>AEEWYFGKITRRESERLLLNPENPRGTFLVRESETTKGAYCLSVSDFDNAKGLNVKHYKIRKLDSGGFYITSRTQFSSLQQLVAYYSKHA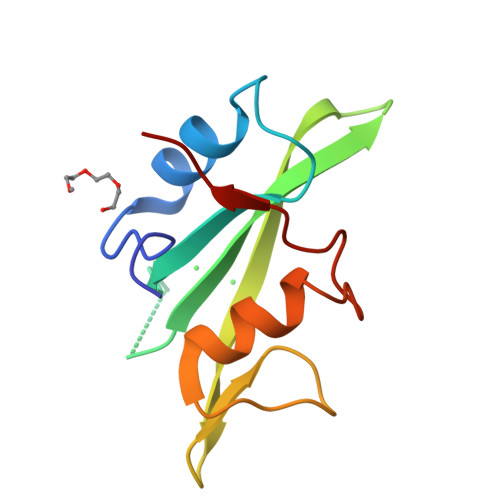DGLCHRLTNVCPT[2x];> PQYEYIPA> SSEDKITVHFINRDGETLTTKGKVGDSLLDVVVENNLDIDGFGACEGTLACSTCHL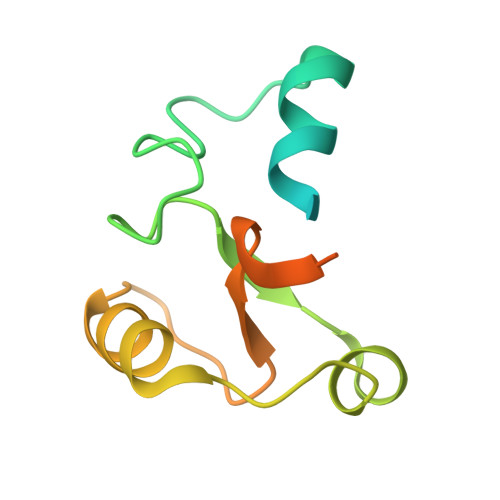IFEDHIYEKLDAITDEENDMLDLAYGLTDRSRLGCQICLTKSMDNMTVRVPETVADAR> MPVTINNFNYNDPIDNNN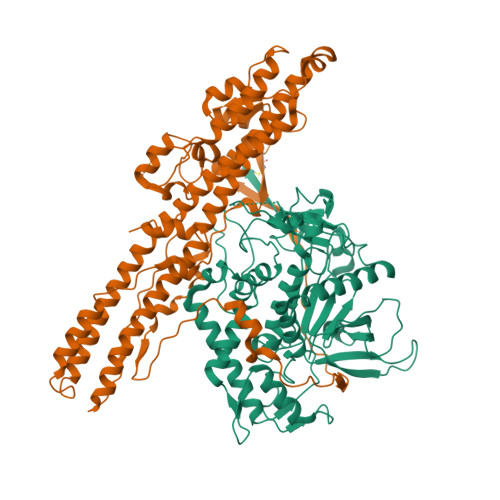IIMMEPPFARGTGRYYKAFKITDRIWIIPERYTFGYKPEDFNKSSGIFNRDVCEYYDPDYLNTNDKKNIFLQTMIKLFNRIKSKPLGEKLLEMIINGIPYLGDRRVPLEEFNTNIASVTVNKLISNPGEVERKKGIFANLIIFGPGPVLNENETIDIGIQNHFASREGFGGIMQMKFCPEYVSVFNNVQENKGASIFNRRGYFSDPALILMHELIHVLHGLYGIKVDDLPIVPNEKKFFMQSTDAIQAEELYTFGGQDPSIITPSTDKSIYDKVLQNFRGIVDRLNKVLVCISDPNININIYKNKFKDKYKFVEDSEGKYSIDVESFDKLYKSLMFGFTETNIAENYKIKTRASYFSDSLPPVKIKNLLDNEIYTIEEGFNISDKDMEKEYRGQNKAINKQAYEEISKEHLAVYKIQMCVDGIITSKTKSLIEGR;> NKALNLQCIDVDNEDLFFIADKNSFSDDLSKNERIEYNTQSNYIENDFPINELILDTDLISKIELPSENTESLTDFNVDVPVYEKQPAIKKIFTDENTIFQYLYSQTFPLDIRDISLTSSFDDALLFSNKVYSFFSMDYIKTANKVVEAGLFAGWVKQIVNDFVIEANKSNTMDKIADISLIVPYIGLALNVGNETAKGNFENAFEIAGASILLEFIPELLIPVVGAFLLESYIDNKNKIIKTIDNALTKRNEKWSDMYGLIVAQWLSTVNTQFYTIKEGMYKALNYQAQALEEIIKYRYNIYSEKEKSNINIDFNDINSKLNEGINQAIDNINNFINGCSVSYLMKKMIPLAVEKLLDFDNTLKKNLLNYIDENKLYLIGSAEYEKSKVNKYLKTIMPFDLSIYTNDTILIEMFNKYNSLEALASGHHHHHH> MLNQSKILTLQAYDPAKVLVFIGGQRVSGFAADTKIVITRNNDNI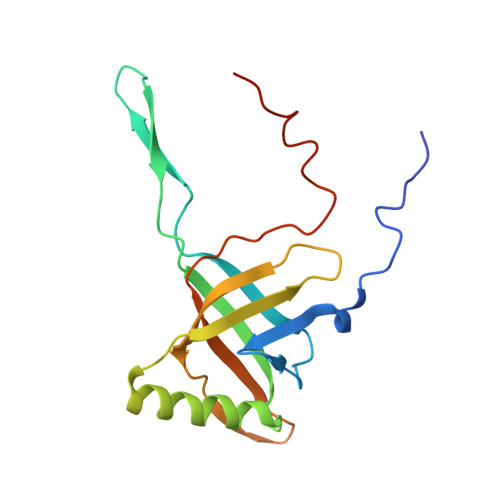SVHAGVDGEISNALSRDNTGVMTLSLQNTAKWNGYLAQWQRQANVTGLIYLPVQVEGSQGLSLNTIGWIQKQPDLSYGTEVGQMDWEIGVLDAWLSPDQIQGIAAGITGLLGLDQ>MAYAQWVIIIIHNVGSQDVKIKNLKASWGKLHADGDKDAEVSASNYEGKIVKPDEKLQINASGRSDAAEGTTGTFDLVDPADGDKQVRHFYWDSPWGSKTNTWTVSGSNTKWMIEYSGQNLDSGALGTITVDTLKKGENLYFQ[4x];>[2x]HHHHHHHHSQAGDTLNDVIQDPTRRNKLINDNNLLKGIIMGRDGPVPSSRELIVRPDTLRAIINNRATIETTTMEAEFTETLMESNYNSASVKVSAPCITANSEYSESSSFKNTETEKSMYTSSRCLFPQGRIDFTTPDSGFDDVIKLSPQFTSGVQAALAKATGTEKREALQNLFQEYGCVFRTKVHIGGVLSAHTMETFSRSENETEVKQDVKAGLEGAVKGWCGGATAGHGNTQGTITTSQNRKLNVKYIVNGGDYTKIQNTEEWVASTNQSEHWRVIEVTEVTAVADLLPQPIRGQVKDLLKPLLGKWVDVEKVPGLESLPVSVYRPKGAIPAGWFWLGDTADASKALLVKPTLPARSGRNPALTSLHQGSGMTEQPFVDLPQYQYLSTYFGSF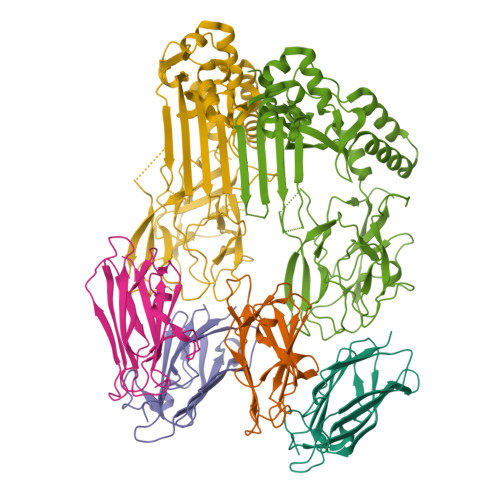AHDTPPGSTLRGLRPDHVLPGRYEMHGDTISTAVYVTRPVDVPFPEDECFDLKSLVRVKLPGSGNPPKPRSALKKSMVLFDSGEK>[2x]MVQPSLPQDDTPDQQEQRNRAIAQQREAYQYSETAGILLIKTLPQSEMFSLKYLIERDKGLVSLIANTLASNIENIFDPFDKLEDFEEMFPLLPKPLVMNTFRNDRVFARQRIAGPNPMVIERVVDKLPDNFPVTDAMFQKIMFTKKTLAEAIAQGKLFITNYKGLAELSPGRYEYQKNGTLVQKTKTIAAPLVLYAWKPEGFGDYRGSLAPIAIQINQQPDPITNPIYTPRDGKHWFIAKIFAQMADGNCHEAISHLARTHLILEPFVLATANELAPNHPLSVLLKPHFQFTLAINELAREQLISAGGYADDLLAGTLEASIAVIKAAIKEYMDNFTEFALPRELARRGVGIGDVDQRGENFLPDYPYRDDAMLLWNAIEVYVRDYLSLYYQSPVQIRQDTELQNWVRRLVSPEGGRVTGLVSNGELNTIEALVAIATQVIFVSGPQHAAVNYPQYDYMAFIPNMPLATYATPPNKESNISEATILNILPPQKLAARQLELMRTLCVFYPNRLGYPDTEFVDVRAQQVLHQFQERLQEIEQRIVLCNEKRLEPYTYLLPSNVPNSTSI

Lipoxygenases (LOX) are key enzymes in the initial step of lipid-mediator biosynthesis. They catalyze a regio- and stereo specific dioxygenation of polyunsaturated fatty acids to yield fatty acid hydroperoxides, which can be further metabolized to a variety of signaling molecules with diverse biological functions. CspLOX2 is the LOX with the highest relative amount of bis-allylic product reported so far, hence it is a suitable candidate to study the molecular basis of the dioxygen positioning at the bis-allylic position. We demonstrate the importance of an active site clamp around the pentadiene system, which fixes the pentadiene during the reaction resulting in 11-HPODE formation.

CspLOX2 crystallized in space group P212121 with one homodimer in the asymmetric unit. As revealed by sequence alignments of CspLOX2 with other LOX12, the N-terminal C2-like domain, which is a common feature of eukaryotic LOX, is absent in CspLOX2. A well-defined boot-shaped channel connects the surface of the protein with its active site. This channel is lined by hydrophobic amino acids and is most likely involved in the positioning of the fatty acid substrate. The catalytic non-heme iron, deeply buried in the CspLOX2 active site, is coordinated by three invariant histidines (His257, His262, His449), Asn453 and the carboxy group of the C-terminal Ile569. The sixth ligand of the octahedrally coordinated iron, which is positioned towards the putative substrate-binding channel, is a water (Fe2+-H2O) or hydroxide molecule (Fe3+-OH) acting as a catalytic base for hydrogen abstraction during catalysis. Besides Leu304, we could identify further crucial residues in the direct environment of the narrow active site that form a clamp-like structure, including Leu258, Ile296, Ala300, Leu502 and Leu506. We also found a putative channel in CspLOX2 at the same position that might serve as oxygen channel as well. This putative channel connects the surface of the protein with the base of the substrate-binding channel at the opposite site of the iron, which is in line with the antarafacial oxidation of the substrate and a high dioxygen concentration at the pro-R face of C-11. Despite extensive efforts, we could not obtain crystals of a CspLOX2 substrate complex.>[2x]SAIENFDAHTPMMQQYLRLKAQHPEILLFYRMGDFYELFYDDAKRASQLLDISLTKRGASAGEPIPMAGIPYHAVENYLAKLVNQGESVAICEQIGDPATSKGPVERKVVRIVTPGTISDEALLQERQDNLLAAIWQDSKGFGYATLDISSGRFRLSEPADRETMAAELQRTNPAELLYAEDFAEMSLIEGRRGLRRRPLWEFEIDTARQQLNLQFGTRDLVGFGVENAPRGLCAAGCLLQYAKDTQ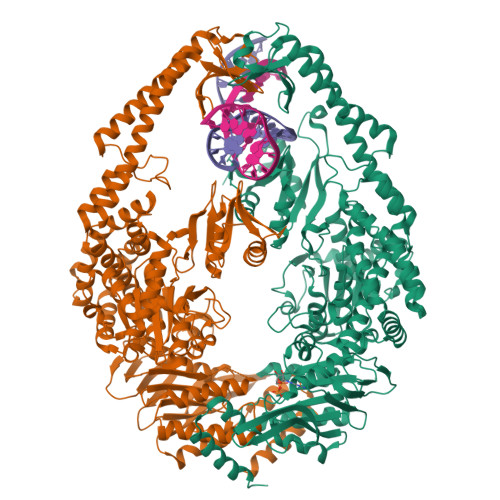RTTLPHIRSITMEREQDSIIMDAATRRNLEITQNLAGGAENTLASVLDCTVTPMGSRMLKRWLHMPVRDTRVLLERQQTIGALQDFTAGLQPVLRQVGDLERILARLALRTARPRDLARMRHAFQQLPELRAQLETVDSAPVQALREKMGEFAELRDLLERAIIDTPPVLVRDGGVIASGYNEELDEWRALADGATDYLERLEVRERERTGLDTLKVGFNAVHGYYIQISRGQSHLAPINYMRRQTLKNAERYIIPELKEYEDKVLTSKGKALALEKQLYEELFDLLLPHLEALQQSASALAELDVLVNLAERAYTLNYTCPTFIDKPGIRITEGRHPVVEQVLNEPFIANPLNLSPQRRMLIITGPNMGGKSTYMRQTALIALMAYIGSYVPAQKVEIGPIDRIFTRVGAADDLASGRSTFMVEMTETANILHNATEYSLVLMNEIGRGTSTYDGLSLAWACAENLANKIKALTLFATHYFELTQLPEKMEGVANVHLDALEHGDTIAFMHSVQDGAASKSYGLAVAALAGVPKEVIKRARQKLRELESIS> MSAIKPDMKIKLRMEGNVNGHHFVIDGDGTGKPFEGKQSMDLEVKEGGPLPFAFDILTTAFAYGNRVF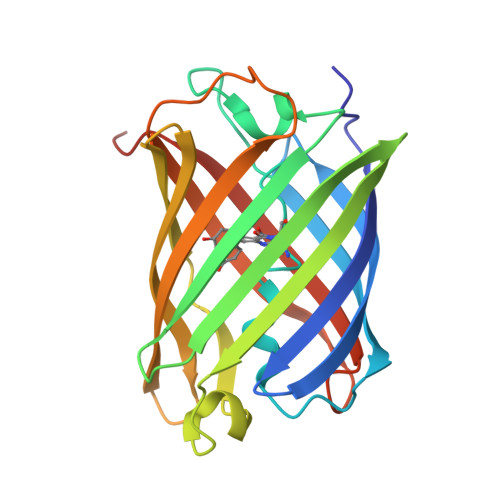AKYPDNIQDYFKQSFPKGYSWERSLTFEDGGICNARNDITMEGDTFYNKVRFYGTNFPANGPVMQKKTLKWEPATEKMYVRDGVLTGDVETALLLEGNAHYRCDFRTTYKAKEKGVKLPGAHFVDHCIEILSHDKDYNKVKLYEHAVAHSGLPDNARR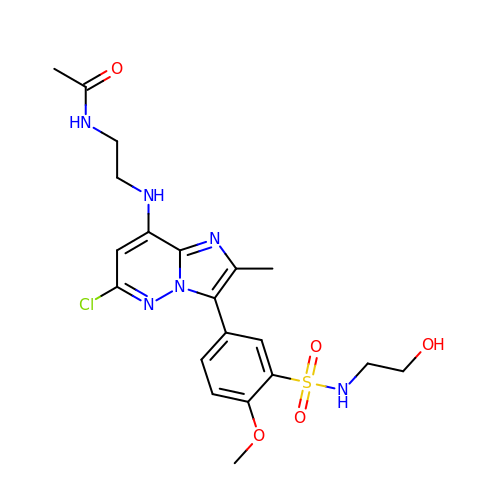~{N}-[2-[[6-chloranyl-3-[3-(2-hydroxyethylsulfamoyl)-4-methoxy-phenyl]-2-methyl-imidazo[1,2-b]pyridazin-8-yl]amino]ethyl]ethanamide | C20 H25 Cl N6 O5 S | MSAKNAXUJISZBR-UHFFFAOYSA-N2-acetamido-3-O-[(1R)-1-carboxyethyl]-2-deoxy-1-O-phosphono-alpha-D-glucopyranose | C11 H20 N 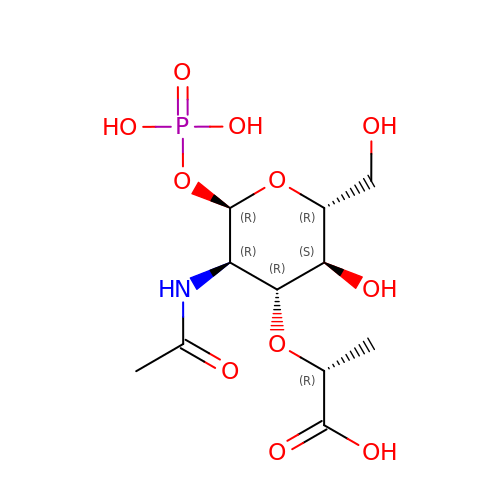O11 P | DTSXRQWOCZUNPL-YVNCZSHWSA-N> SGDMADAFGDELFSVFEGDSTTAAGTKKDKEKDKGKWKGPPGSADKAGKRFDGKLQSESTNNGKNKRDVDFEGTDEPIFGKKPRIEESITEDLSLADLMPRVKVQSVETVEGCTHEVALPAEEDYLPLKPRVGKAAKEYPFILDAFQREAIQCVDNNQSVLVSAHTSAGKTVCAEYAIALALREKQRVIFTSPIKALSNQKYREMYEEFQDVGLMTGDVTINP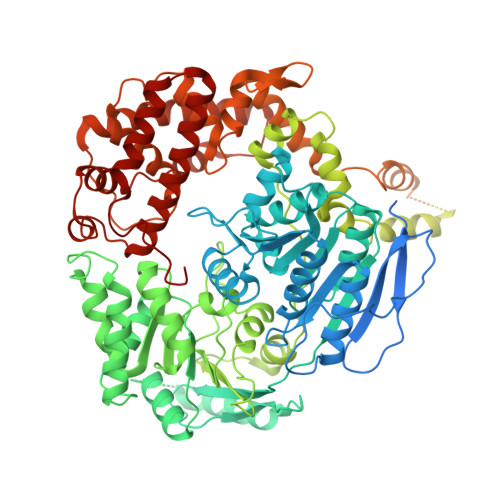TASCLVMTTEILRSMLYRGSEVMREVAWVIFDEIHYMRDSERGVVWEETIILLPDNVHYVFLSATIPNARQFAEWICHLHKQPCHVIYTDYRPTPLQHYIFPAGGDGLHLVVDENGDFREDNFNTAMQVLRDAGDLAKGDQKGRKGGTKGPSNVFKIVKMIMERNFQPVIIFSFSKKDCEAYALQMTKLDFNTDEEKKMVEEVFSNAIDCLSDEDKKLPQVEHVLPLLKRGIGIHHGGLLPILKETIEILFSEGLIKALFATETFAMGINMPARTVLFTNARKFDGKDFRWISSGEYIQMSGRAGRRGMDDRGIVILMVDEKMSPTIGKQLLKGSADPLNSAFHLTYNMVLNLLRVEEINPEYMLEKSFYQFQHYRAIPGVVEKVKNSEEQYNKIVIPNEESVVIYYKIRQQLAKLGKEIEEYIHKPKYCLPFLQPGRLVKVKNEGDDFGWGVVVNFSKKSNVKPNSGELDPLYVVEVLLRCSKESLKNSATEAAKPAKPDEKGEMQVVPVLVHLLSAISSVRLYIPKDLRPVDNRQSVLKSIQEVQKRFPDGIPLLDPIDDMGIQDQGLKKVIQKVEAFEHRMYSHPLHNDPNLETVYTLCEKKAQIAIDIKSAKRELKKARTVLQMDELKCRKRVLRRLGFATSSDVIEMKGRVACEISSADELLLTEMMFNGLFNDLSAEQATALLSCFVFQENSSEMPKLTEQLAGPLRQMQECAKRIAKVSAEAKLEIDEETYLSSFKPHLMDVVYTWATGATFAHICKMTDVFEGSIIRCMRRLEELLRQMCQAAKAIGNTELENKFAEGITKIKRDIVFAASLYL> MKKLVMTAAVAAILGAASP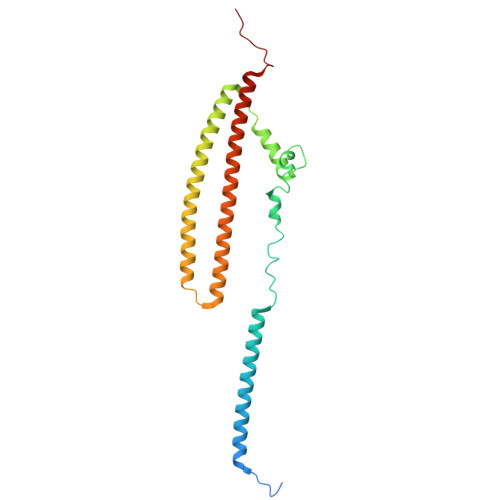VMAQGIPVFDGTRALDFVQQFARMKEQLDTAKDQLAEAQRMYEAVTGGRGLGDLMRNAQLREYLPDDLRTVYDSANGGGYSGISGSINDILRDERLNGSVADMRRSIEERSRTAAATDKAVGLRAYEGAQQRLAQIEGLMDEISRTQDQKAIEELQARIAGEQAAIQNETTKLQMIAQLRQAEQALISEQRRERNMRILSSGNQGMPTIQ>GDKDCEMKRTTLDSPLGKLELSGCEQGLHRIIFLGKGTSAADAVEVPAPAAVLGGPEPLMQATAWLNAYFHQPEAIEEFPVPALHHPVFQQESFTRQVLWKLLKVVKFGEVISYSHLAALAGNPAATAAVKTALSGNPVPILIPCHRVVQGDLDVGGYEGGLAVKEWLLAHEGHRLGKPGLGGSLEVLFQGPDYDIPTTLEVLFQGPANGTADVRKLFIFTTTQNYFGLMSELWDQPLLCNCLEINNFLDDGNQMLLRVQRSDAGISFSNTIEFGDTKDKVLVFFKLRPEVITDENLHDNILVSSMLESPISSLYQAVRQVFAPMLLKDQEWSRNFDPKLQNLLSELEAGLGIVLRRSDTNLTKLKFKEDDTRGILTPSDEFQFWIEQAHRGNKQISKERANYFKELFETIAREFYNLDSLSLLEVVDLVETTQDVVDDVWRQTEHDHYPESRMLHLLDIIGGSFGRFVQKKLGTLNLWEDPYYLVKESLKAGISICEQWVIVCNHLTGQVWQRYVPHPWKNEKYFPETLDKLGKRLEEVLAIRTIHEKFLYFLPASEEKIICLTRVFEPFTGLNPVQYNPYTEPLWKAAVSQYEKIIAPAEQKIAGKLKNYISEIQDSPQQLLQAFLKYKELVKRPTISKELMLERETLLARLVDSIKDFRLDFENRCRGIPGDASGPLSGKNLSEVVNSIVWVRQLELKVDDTIKIAEALLSDLPGFRCFHQSAKDLLDQLKLYEQEQFDDWSRDIQSGLSDSRSGLCIEASSRIMELDSNDGLLKVHYSDRLVILLREVRQLSALGFVIPAKIQQVANIAQKFCKQAIILKQVAHFYNSIDQQMIQSQRPMMLQSALAFEQIIKNSKAGSGGKSQITWDNPKELEGYIQKLQNAAERLATENRKLRKWHTTFCEKVVVLMNIDLLRQQQRWKDGLQELRTGLATVEAQGFQASDMHAWKQHWNHQLYKALEHQYQMGLEALNENLPEINIDLTYKQGRLQFRPPFEEIRAKYYREMKRFIGIPNQFKGVGEAGDESIFSIMIDRNASGFLTIFSKAEDLFRRLSAVLHQHKEWIVIGQVDMEALVEKHLFTVHDWEKNFKALKIKGKEVERLPSAVKVDCLNINCNPVKTVIDDLIQKLFDLLVLSLKKSIQAHLHEIDTFVTEAMEVLTIMPQSVEEIGDANLQYSKLQERKPEILPLFQEAEDKNRLLRTVAGGGLETISNLKAKWDKFELMMESHQLMIKDQIEVMKGNVKSRLQIYYQELEKFKARWDQLKPGDDVIETGQHNTLDKSAKLIKEKKIEFDDLEVTRKKLVDDCHHFRLEEPNFSLASSISKDIESCAQIWAFYEEFQQGFQEMANEDWITFRTKTYLFEEFLMNWHDRLRKVEEHSVMTVKLQSEVDKYKIVIPILKYVRGEHLSPDHWLDLFRLLGLPRGTSLEKLLFGDLLRVADTIVAKAADLKDLNSRAQGEVTIREALRELDLWGVGAVFTLIDYEDSQSRTMKLIKDWKDIVNQVGDNRCLLQSLKDSPYYKGFEDKVSIWERKLAELDEYLQNLNHIQRKWVYLEPIFGRGALPKEQTRFNRVDEDFRSIMTDIKKDNRVTTLTTHAGIRNSLLTILDQLQRCQRSLNEFLEEKRSAFPRFYFIGDDDLLEILGQSTNPSVIQSHLKKLFAGINSVCFDEKSKHITAMKSLEGEVVPFKNKVPLSNNVETWLNDLALEMKKTLEQLLKECVTTGRSSQGAVDPSLFPSQILCLAEQIKFTEDVENAIKDHSLHQIETQLVNKLEQYTNIDTSSEDPGNTESGILELKLKALILDIIHNIDVVKQLNQIQVHTTEDWAWKKQLRFYMKSDHTCCVQMVDSEFQYTYEYQGNASKLVYTPLTDKCYLTLTQAMKMG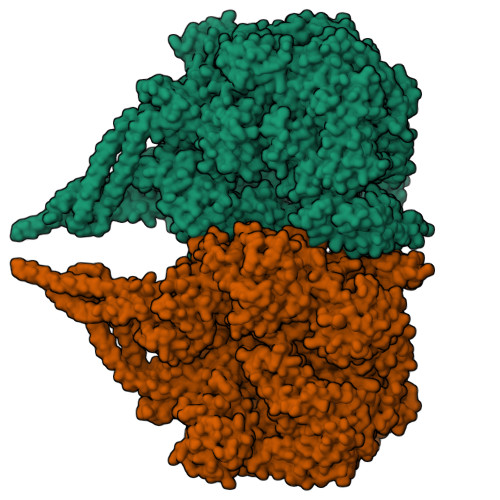LGGNPYGPAGTGKTESVKALGGLLGRQVLVFNCDEGIDVKSMGRIFVGLVKCGAWGCFDEFNRLEESVLSAVSMQIQTIQDALKNHRTVCELLGKEVEVNSNSGIFITMNPAGKGYGGRQKLPDNLKQLFRPVAMSHPDNELIAEVILYSEGFKDAKVLSRKLVAIFNLSRELLTPQQHYDWGLRALKTVLRGSGNLLRQLNKSGTTQNANESHIVVQALRLNTMSKFTFTDCTRFDALIKDVFPGIELKEVEYDELSAALKQVFEEANYEIIPNQIKKALELYEQLCQRMGVVIVGPSGAGKSTLWRMLRAALCKTGKVVKQYTMNPKAMPRYQLLGHIDMDTREWSDGVLTNSARQVVREPQDVSSWIICDGDIDPEWIESLNSVLDDNRLLTMPSGERIQFGPNVNFVFETHDLSCASPATISRMGMIFLSDEETDLNSLIKSWLRNQPAEYRNNLENWIGDYFEKALQWVLKQNDYVVETSLVGTVMNGLSHLHGCRDHDEFIINLIRGLGGNLNMKSRLEFTKEVFHWARESPPDFHKPMDTYYDSTRGRLATYVLKKPEDLTADDFSNGLTLPVIQTPDMQRGLDYFKPWLSSDTKQPFILVGPEGCGKGMLLRYAFSQLRSTQIATVHCSAQTTSRHLLQKLSQTCMVISTNTGRVYRPKDCERLVLYLKDINLPKLDKWGTSTLVAFLQQVLTYQGFYDENLEWVGLENIQIVASMSAGGRLGRHKLTTRFTSIVRLCSIDYPEREQLQTIYGAYLEPVLHKNLKNHSIWGSSSKIYLLAGSMVQVYEQVRAKFTVDDYSHYFFTPCILTQWVLGLFRYDLEGGSSNHPLDYVLEIVAYEARRLFRDKIVGAKELHLFDIILTSVFQGDWGSDILDNMSDSFYVTWGARHNSGARAAPGQPLPPHGKPLGKLNSTDLKDVIKKGLIHYGRDNQNLDILLFHEVLEYMSRIDRVLSFPGGSLLLAGRSGVGRRTITSLVSHMHGAVLFSPKISRGYELKQFKNDLKHVLQLAGIEAQQVVLLLEDYQFVHPTFLEMINSLLSSGEVPGLYTLEELEPLLLPLKDQASQDGFFGPVFNYFTYRIQQNLHIVLIMDSANSNFMINCESNPALHKKCQVLWMEGWSNSSMKKIPEMLFSETGGGEKYNDKKRKEEKKKNSVDPDFLKSFLLIHESCKAYGATPSQYMTFLHVYSAISSSKKKELLKRQSHLQAGVSKLNEAKALVDELNRKAGEQSVLLKTKQDEADAALQMITVSMQDASEQKTELERLKHRIAEEVVKIEERKNKIDDELKEVQPLVNEAKLAVGNIKPESLSEIRSLRMPPDVIRDILEGVLRLMGIFDTSWVSMKSFLAKRGVREDIATFDARNISKEIRESVEELLFKNKGSFDPKNAKRASTAAAPLAAWVKANIQYSHVLERIHPLETEQAGLESNLKKTEDRKRKLEELLNSVGQKVSELKEKFQSRTSEAAKLEAEVSKAQETIKAAEVLINQLDREHKRWNAQVVEITEELATLPKRAQLAAAFITYLSAAPESLRKTCLEEWTKSAGLEKFDLRRFLCTESEQLIWKSEGLPSDDLSIENALVILQSRVCPFLIDPSSQATEWLKTHLKDSRLEVINQQDSNFITALELAVRFGKTLIIQEMDGVEPVLYPLLRRDLVAQGPRYVVQIGDKIIDYNEEFRLFLSTRNPNPFIPPDAASIVTEVNFTTTRSGLRGQLLALTIQHEKPDLEEQKTKLLQQEEDKKIQLAKLEESLLETLATSQGNILENKDLIESLNQTKASSALIQESLKESYKLQISLDQERDAYLPLAESASKMYFIISDLSKINNMYRFSLAAFLRLFQRALQNKQDSENTEQRIQSLISSLQHMVYEYICRCLFKADQLMFALHFVRGMHPELFQENEWDTFTGVVVGDMLRKADSQQKIRDQLPSWIDQERSWAVATLKIALPSLYQTLCFEDAALWRTYYNNSMCEQEFPSILAKKVSLFQQILVVQVLRPDRLQSAMALFACKTLGLKEVSPLPLNLKRLYKETLEIEPILIIISPGADPSQELQELANAERSGECYHQVAMGQGQADLAIQMLKECARNGDWLCLKNLHLVVSWLPVLEKELNTLQPKDTFRLWLTAEVHPNFTPILLQSSLKITYESPPGLKKNLMRTYESWTPEQISKKDNTHRAHALFSLAWFHAACQERRNYIPQGWTKFYEFSLSDLRAGYNIIDRLFDGAKDVQWEFVHGLLENAIYGGRIDNYFDLRVLQSYLKQFFNSSVIDVFNQRNKKSIFPYSVSLPQSCSILDYRAVIEKIPEDDKPSFFGLPANIARSSQRMISSQVISQLRILGRSITAGSKFDREIWSNELSPVLNLWKKLNQNSNLIHQKVPPPNDRQGSPILSFIILEQFNAIRLVQSVHQSLAALSKVIRGTTLLSSEVQKLASALLNQKCPLAWQSKWEGPEDPLQYLRGLVARALAIQNWVDKAEKQALLSETLDLSELFHPDTFLNALRQETARAVGRSVDSLKFVASWKGRLQEAKLQIKISGLLLEGCSFDGNQLSENQLDSPSVSSVLPCFMGWIPQDACGPYSPDECISLPVYTSAERDRVVTNIDVPCGGNQDQWIQCGAALFLKNQ[2x]>SNAAGMFRALFRQAVEDDRYGEFLDVLAEASAFRPQFASPEACSERLDPVLLAGGPTDRAEGRAVLVGCTGTAANGGPHEFLRLSTSFQEERDFLAVPLPGYGTGTGTGTALLPADLDTALDAQARAILRAAGDAPV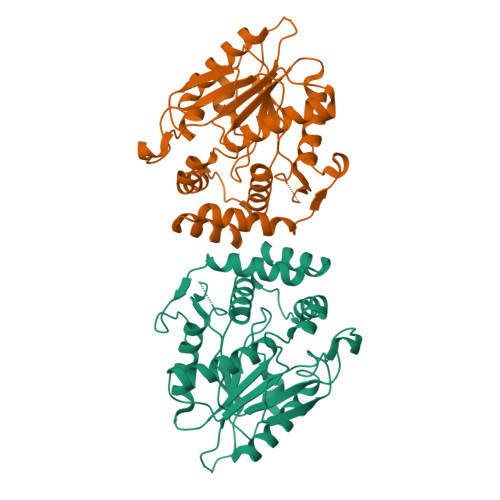VLLGHSGGALLAHELAFRLERAHGAPPAGIVLVDPYPPGHQEPIEVWSRQLGEGLFAGELEPMSDARLLAMGRYARFLAGPRPGRSSAPVLLVRASEPLGDWQEERGDWRAHWDLPHTVADVPGDHFTMMRDHAPAVAEAVLSWLDAIEGIEGAGK[2x]2-METHYLACETOACETYL COA 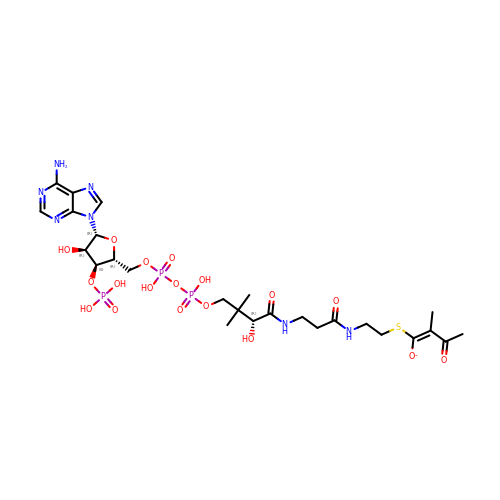| C26 H41 N7 O18 P3 S | HJBMSIYWKRMJGR-LURNCBTNSA-M5-amino-2,4,6-triiodobenzene-1,3-dicarboxylic acid | C8 H4 I3 N O4 | 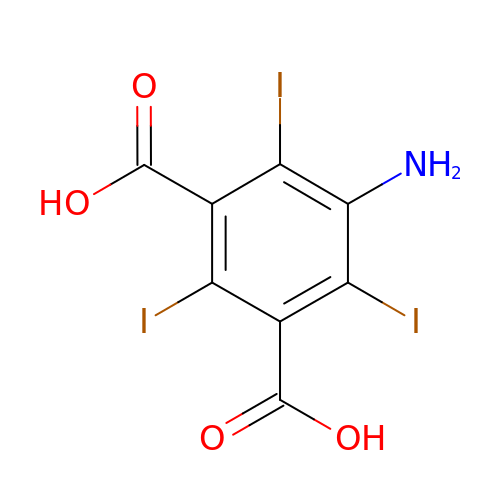JEZJSNULLBSYHV-UHFFFAOYSA-N>GPHMKTHIDDYSTWDIVKATQYGIYERCRELVEAGYDVRQPDKANVTLLHW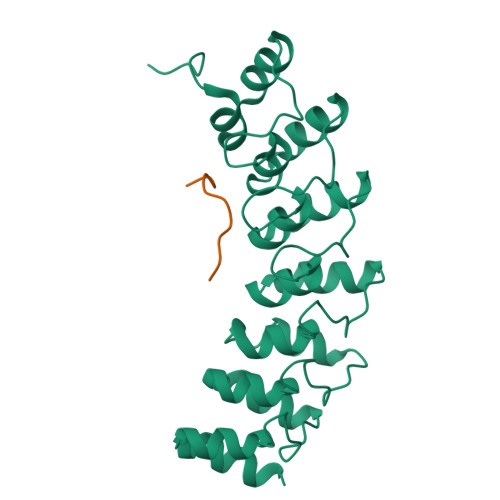AAINNRIDLVKYYISKGAIVDQLGGDLNSTPLHWATRQGHLSMVVQLMKYGADPSLIDGEGCSCIHLAAQFGHTSIVAYLIAKGQDVDMMDQNGMTPLMWAAYRTHSVDPTRLLLTFNVSVNLGDKYHKNTALHWAVLAGNTTVISLLLEAGANVDAQNIKGESALDLAKQRKNVWMINHLQEARQAK[2x];>[2x]GVVASQPARV> GLPIDLRGKRAFIAGIADDNGYGWAVAKSLAAAGAEILVGTWVPALNIFETSLRRGKFDQSRVLPDGSLMEIKKVYPLDAVFDNPEDVPEDVKANKRYAGSSNWTVQEAAECVRQDFGSIDILVHSLANGPEVSKPLLETSRKGYLAAISASSYSFVSLLSHFLPIMNPGGASISL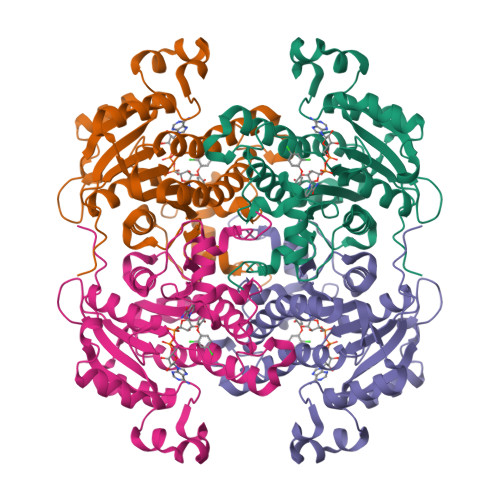TYIASERIIPGYGGGMSSAKAALESDTRVLAFEAGRKQNIRVNTISAGPLGSRAAKAIGFIDTMIEYSYNNAPIQKTLTADEVGNAAAFLVSPLASAITGATIYVDNGLNSMGVALDSPVF>GSSSRECSYCGKFFRSNYYLNIHLRTHTGEKPY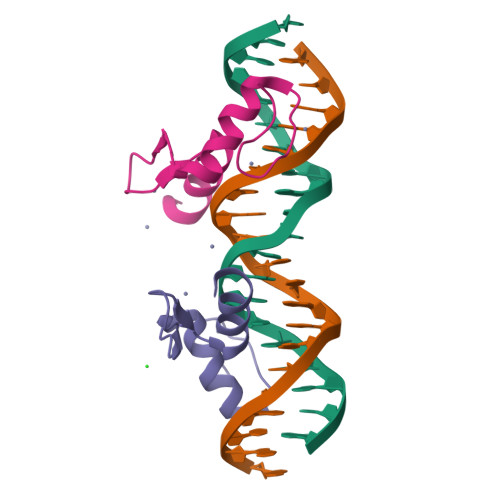KCEFCEYAAAQKTSLRYHLERHHK[2x]> GPNPYERGPDPTEDSIEAIRGPFSVATERVSSFASGFGGGTIYYPRETDEGTFGAVAVAPGFTASQGSMSWYGERVASHGFIVFTIDTNTRLDAP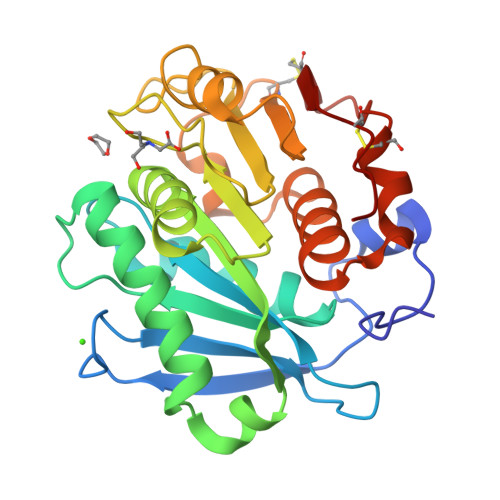GQRGRQLLAALDYLVERSDRKVRERLDPNRLAVMGHAMGGGGSLEATVMRPSLKASIPLTPWHLDKTWGQVQVPTFIIGAELDTIAPVSTHAKPFYESLPSSLPKAYMELCGATHFAPNIPNTTIAKYVISWLKRFVDEDTRYSQFLCPNPTDRAICEYRSTCPYKLN The adenosine triphosphate (ATP)-binding cassette (ABC) importer GlnPQ from Lactococcus lactis has two sequential covalently linked substrate-binding domains (SBDs), which capture the substrates and deliver them to the translocon. GlnPQ is an ABC transporter involved in the uptake of glutamine, glutamic acid, and asparagine and was found to be a robust model protein to study the mechanism of substrate delivery from SBDs to the translocon. SBDs operate in a Venus-fly trap mechanism, where the binding site for a substrate is located between two lobes of an SBD, which is connected by two antiparallel β-strands (the hinge region). We report three high-resolution structures of SBD1, namely, the wild-type SBD1 with bound asparagine or arginine, and E184D SBD1 with glutamine bound.

In addition, arginine binds in the substrate pocket but is not transported by GlnPQ. The effect of nontransported substrates on substrate affinity was shown using FRET measurements, where arginine, histidine, and lysine can competitively inhibit the uptake of glutamine (via SBD1 and SBD2) and asparagine (via SBD1).35 To investigate this inhibitory effect, we aimed to obtain the crystal structure of arginine bound to SBD1. Unfortunately, we failed to obtain well-diffracting SBD1-Arg crystals; hence, we soaked crystals of the unliganded SBD1 with 10 mM arginine. In the obtained crystal structure, there are two molecules of SBD1 in the asymmetric unit cell, which show a slightly different binding pattern of arginine. Most interactions are with the large subdomain and the carboxyl-side chain of E184, which makes a hydrogen bond to the α-amino group of the Arg. Similar to the binding of the high-affinity substrate asparagine, the α-carboxyl group of arginine is stabilized by a salt bridge with R101 and hydrogen bonds to the backbone nitrogen and the hydroxyl group of T96. Clearly, the bound arginine traps SBD1 in a conformation that is unable to close, hence explaining the inability of GlnPQ to transport arginine leading to the inhibition of the transport of Gln and Asn. It is also notable that this binding does not affect the global rearrangement of the protein structure. Furthermore, partial domain closure has also been demonstrated for ligand-binding domains of ionotropic glutamate receptors iGluRs. Together with the fact that also in solution arginine prevents closure of SBD1,35 we believe that our observation that arginine is incapable of triggering the conformational change is correct. The presence of l-arginine and l-histidine at the binding site leads to the inability of SBDs to close fully hence leading to the loss of transport activity of the transporter.

>[2x]ETTVKIASDSSYAPFEFQNGQKKWVGIDVDIMQEVAKINDWKLEMSYPGFDAALQNLKAGQVDGIIAGMTITDERKETFDFSNPYYTSALTIATTKDSKLSDYSDLKGKAVGAKNGTAAQTWLQENQKKYGYTIKTYSDGVHMFAALSSGNIAGAMDEVPVISYAMKQGQDLAMNFPSISLPGGYGFAVMKGKNSTLVDGFNKALAEMKSNGDYDKILKKYGITA BlaR1 and MecR1 are membrane proteins with an N-terminal zinc metalloprotease domain and a C-terminal extracellular β-lactam-binding sensor domain. β-Lactam binding to the extracellular BlaR1 sensor domain regulates BlaI cleavage by the zinc metalloprotease domain in the cytoplasm. BlaR1 forms a domain-swapped dimer, with the zinc metalloprotease active site accessible from the cytoplasm. BlaR1 undergoes spontaneous autocleavage in cis between Ser283 and Phe284 and we describe the catalytic mechanism and specificity underlying the self and BlaI cleavage.

An asymmetric homodimer class was identified, resulting in a reconstruction of the previously uncharacterized BlaR1(WT) transmembrane and zinc metalloprotease region to 3.8 Å with a local resolution extending to about 3.3 Å. Dimerization defines a central cavity, which in the native membrane is presumably filled with lipids. Densities consistent with phosphatidylglycerol headgroups are observed lining the electropositive surface formed at the base of the cavity. The loop connecting helices α8 and swapped α9, housing the scissile bond between residues Ser283 and Phe284 (residues 271 to 289; here termed the autocleavage loop), enters the zinc metalloprotease active site of its own chain, directly demonstrating that autocleavage occurs in cis. The initial zinc metalloprotease substrate, the autocleavage loop captured here in uncleaved and cleaved states, provides insights into the molecular details of substrate specificity. The P4–P1′ residues of the autocleavage loop (Leu280, Ser281, His282, Ser283, Phe284) adopt the typical β-strand conformation of protease substrates, which runs anti-parallel to β3 of the gluzincin domain β-sheet analogous to substrate binding in thermolysin related proteases. In addition to main-chain β-strand hydrogen bonds between Thr172 and His282, the substrate is anchored by hydrophobic interactions of Leu280 into the S4 pocket at one end and P1′ Phe284 inserting into the S1′ subsite at the other, with the intervening P2 His282 within the S2 pocket the other important specificity determinant. In the WT structure, one chain shows clear separation of Ser283(P1) and Phe284(P1′) supporting a post-autocleavage state. By contrast, the density in the alternate chain is more uninterrupted, suggesting a pre-cleavage state, consistent with a population of both uncleaved and cleaved protein in the sample used for cryo-EM. The autocleavage loop is in the approximate position for cleavage, with the P1 Ser283 carbonyl orientated favourably towards the catalytic zinc, which canonically acts to polarize the scissile bond, promoting its electrophilicity and subsequent nucleophilic attack by an activated water to promote cleavage.

>[3x]MAKLLIMSIVSFCFIFLLLLFFRYILKRYFNYMLNYKVWYLTLLAGLIPFIPIKFSLFKFNNVNNQAPTVESKSHDLNHNINTTKPIQEFATDIHKFNWDSIDNICTVIWIVLVIILSFKFLKALLYLKYLKKQSLYLNENEKNKIDTILFNHQYKKNIVIRKAETIQSPITFWYGKYIILIPSSYFKSVIDKRLKYIILHEYAHAKNRDTLHLIIFNIFSIIMSYNPLVHIVKRKIIHDNEVEADRFVLNNINKNEFKTYAESIMDSVLNVPFFNKNILSHSFNGKKSLLKRRLINIKEANLKKQSKLILIFICIFTFLLMVIQSQFLMGQSITDYNYKKPLHNDYQILDKSKIFGSNSGSFVMYSMKKDKYYIYNEKESRKRYSPNSTYKIYLAMFGLDRHIINDENSRMSWNHKHYPFDAWNKEQDLNTAMQNSVNWYFERISDQIPKNYTATQLKQLNYGNKNLGSYKSYWMEDSLKISNLEQVIVFKNMMEQNNHFSKKAKNQLSSSLLIKKNEKYELYGKTGTGIVNGKYNNGWFVGYVITNHDKYYFATHLSDGKPSGKNAELISEKILKEMGVLNGQELALVPRGSSAHHHHHH> MPVDFTGYWKMLVNENFEEYLRALDVNVALRKIANLLKPDLEIVQDGDHMIIRTLSTFRNYIMDFQVGKEFEEDLTGIDDRKCMTTVSWDGDKLQC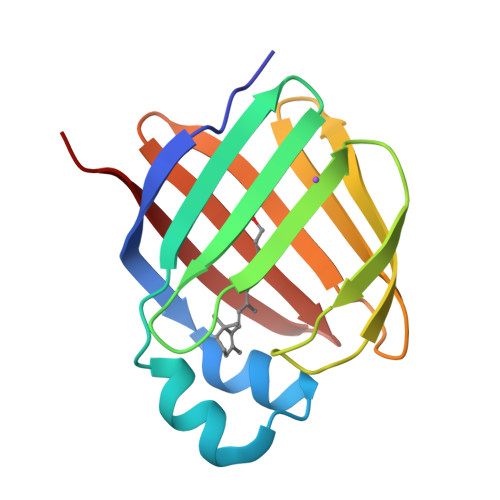VQKGEKEGRGWTQWIEGDELHLEMRVEGVVCKQVFKKVQ> DKTALTVIRLGGIFSRRQQYQLPVNVTASTLTLLLQKPLKLHDMEVVHISFERSALEQW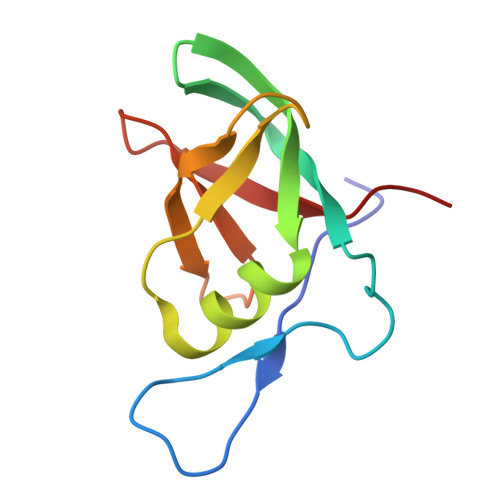LSKGGEIRGKLNGIGFAQKLNLEVDSAQHLVVRDVSLQGSTLALPGS>[4x]MTTQAPTFTQPLQSVVVLEGSTATFEAHISGFPVPEVSWFRDGQVISTSTLPGVQISFSDGRAKLTIPAVTK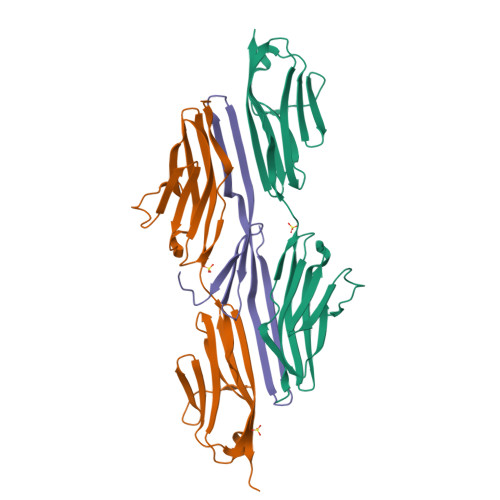ANSGRYSLKATNGSGQATSTAELLVKAETAPPNFVQRLQSMTVRQGSQVRLQVRVTGIPTPVVKFYRDGAEIQSSLDFQISQEGDLYSLLIAEAYPEDSGTYSVNATNSVGRATSTAELLVQGETREEF;>MATSELSSEVSEENSERREAFWAEWKDLTLSTRPEEGSSLHEEDTQRHETYHQQGQSQVLVQRSPWLMMRMGILGRGLQEYQLPYQRVLPLPIFTPAKMGATKEEREDTPIQLQELLALETALGGQSVDRQEVAEITKQLPPVVPVSKPGALRRSLSRSMSQEAQRG[2x]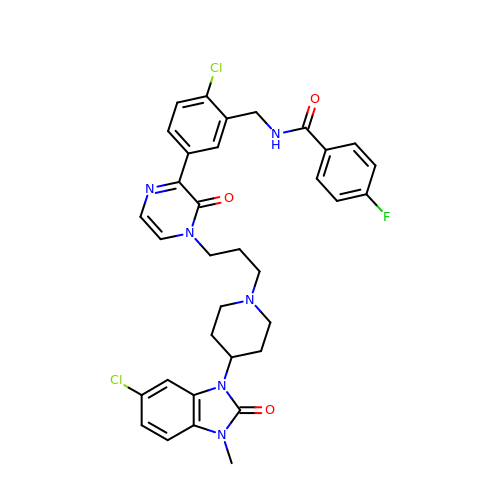N-{[2-chloro-5-(4-{3-[4-(6-chloro-3-methyl-2-oxo-2,3-dihydro-1H-benzimidazol-1-yl)piperidin-1-yl]propyl}-3-oxo-3,4-dihydropyrazin-2-yl)phenyl]methyl}-4-fluorobenzamide | C34 H33 Cl2 F N6 O3 | MNEPYBOQUOAGHK-UHFFFAOYSA-N>[22x]MSGTEEAILGGRDSHPAAGGGSVLCFGQCQYTAEEYQAIQKALRQRLGPEYISSRMAGGGQKVCYIEGHRVINLANEMFGYNGWAHSITQQNV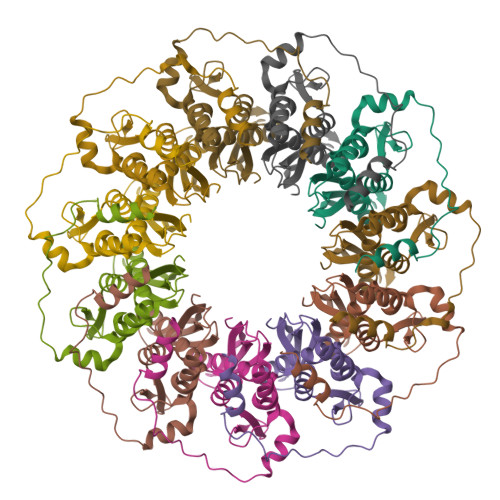DFVDLNNGKFYVGVCAFVRVQLKDGSYHEDVGYGVSEGLKSKALSLEKARKEAVTDGLKRALRSFGNALGNCILDKDYLRSLNKLPRQLPLEVDLTKAKRQDLEPSVEEARYNSCR> MSYSAYFAKAGFQFPAGLSALVAGIVALNVCTGRPTKGTKEISNAEYNATPIGYLQSPDQHPTAFPKVPGMKDVHGSPHHHH;> MMRAAQKAKQELPATVLTQTRSYLAPLRSDFTEEITAPKVASASNLVNEWNNKKQATENLMKLLQAYKDIGDAKSEPLLKNHNPRTFEDRDYPVPDFRTQNLKAGDVPKFFDTVISTRASAAIASKDKFWAGRKTEAEAASAKASAAFPRVAVPEWKKGKTVSIENLNTVTDKYAAALVPKRKLALPVLPEGVKKAVEDFAASVGQAKNASEVSELLAKSLAEKAVVTEGGKVVEGFSYVSKAVAAKVIATRRAEVHERLLKLWAKRLLVSPELAIVPLNEFDAQLASKFEGISPKYQELLSAVAQGNKTFAQRLNSSPAFSSFLLKREKAESEVPPSELELEAAQKAAELEDPEVALRTLLGPQMEALGASDLLLSEQIRVITEHRYTPDRLQYKEGMKLADKIAAQEAALKEELKVIYGDNVDVKHFQASPRTPVQQLFDSLKNAAANKERAAKEAAAAASPYLAYAVTKKQEVQADPSNIPFDEVLYPQLSEELLELELSDIREDEIALEKAEEEELWLLTLTQQFKHIQKHFGIDLPHSVVAHMDPLLIKKIDWETTNALEDFDITLDDMGAEDAKEQWGAENLSHHFLPLIRYRRDLARKNGDRYGPDLVNGN;> ENDVPAILKEIDSLVSREAVSAKEVSDAAVALTYLQVKANRRLWGKVLEKAGAAQDYDAASLTNLLWAINTGGVEHFKTVAELAGPAVSLLPSLSPVQLSIVVEALGGAGVKNYELYNKASAVVVSKIGEFKPAEIARVLYGVAFGGVNDVALAKAAGKVFASTEVDSRTAAQALYALAKLGRADKATVDALLKSFKKGTESASDAAAASFALGSLSFKAEKAIVDALKASAGDLAPAQAVEAAYGLALSGATDAEAFKALFGVVAPAIEKAPDALEVSSLAQLHVASTISGAKLPAAVGSFVAKAFGLAADAARLKRSSAESALVADVAAATAVAFGAQYRPEVASAVASYVKTAPDGSVLDIAITKGDAKVLVQAVPSSLLTSTTPAKPLGHVAAYSKVREAQGYAVAVVPANEFEALPDQKAKAQYVLAAIKKVAPSF;> MRQASRLALSIRQAGNVEAASAVPAMTRQFSAPGSHEHHETPLSKVMPTVVSIPRKVACLALGATKKVVCGLASSGPSQNLVSTFANKVIVEENLVNVAEIDVPFWSYWLSSAGFTSKDAFVKFAEAVKPKVAALSTSDITNLTVAFKRANYYDKDLFTGIEANVSANFTKFETEQLLQIVATFDAFNHSSVAFLDDVADSITYCNHYLAPVRAGADELATLLTYYAKNGHERADLLATVARGFSEVSLGKLSAAQRKDTVLSALKAFQTFGFYPESIEAVIGAALVSPAEYSAEELKEVEAVKVAAENALGGEFVLIQEGAHGH;> ATEPAVSKKEVLYFLSSKDAESSTAVKSYLKSLYAGAQVEATETDASELIAQLEKKYLSAQVVEPGVHNIALPLGESGSAPVKRYAAELFNLGAQAGFECPFIEVSKKFGQETATSETVKDVLNKTKSYVSADYNAALNEVLSSVEAEINGPVLFDGKTEGFKKFAAKAKAVAVSRGLPADTILAYCAGSANEDAADKVSKEFFTWFESAYTADAAAEVKAIEAEAASILDRHLAKPVAQIRKEQASAYASLLKRAETAKGAKWAEKYLEDVKAVQWFDASVAEAPASGPKVAA;> MKLLPESLQQEAATAAVVASWVLWHLDTQLLPTIMREHKLHACWAAAAKRYNEKLFKLNPSYDRVLSLPAVSKNQVLENVFHTAPKAPVEHLEKMVSANSKVYDALNLQSKRVLIWQVKPALF;> MMLRTLTRSSAVAGQAVRLFKTSAAAAEGNSVAGIIKSVNETSGANLLSSLKTIKAQAAPIYPAAASSTGYSTQAKIALFGALSWILYRADGQSKAHEWIVDLNLNVLQAAWLISFSSLIPFRAVYFAFRGMAPAT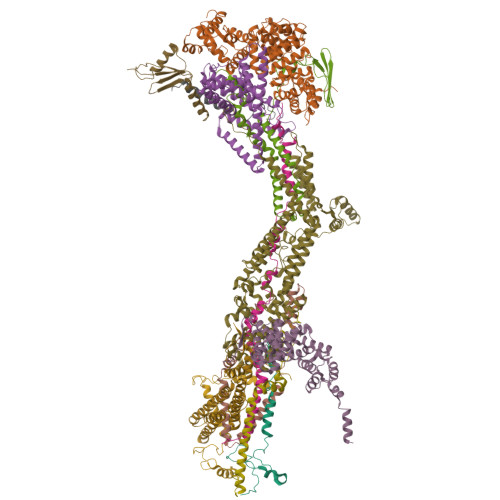ASTLNGLKTFSSISL;> MSSVRAGVEAGRRDLTTFTFSGLQDAPVAALSGSIKLNVAAKAGKAEVTVAAGAAKAATQVSAAALRKLSGSKISLAEVARISVLHSSIQNYLLSLSNERYQLLSQWPDFTTMYGKDFYYRAHPEDLKKFYDAADEYYKLYETVTEFDSLSALASQVVPNYAARRRSTVHPAIGSTVADGAFTNFLLSKQ;> MVLGEVYLKDILRTPPTGAIPANVPHPFQTSFYTYATKKLIPRHWYLLGGFTFTITLYGILDGLRDSGKKKAYDEAIHAGKTPYTAGGH;> MAVTSFLGKAFEKYFYDFSAYEQFGLNRFLSSKGQYVALRHVGFVMVGVNVLLAANFPFNPPFPTIGMCPAGWEGTWVCQADKAKALEMYKEWKKSN;> MSVLSSVSMGSRIGSSLLGRSSAYLAQCGFSTRSNLNGSIDTSSSVFQALSSDNENKPAASPLNVKLPGMSCSSILLPKTSRIAVPFGNQTMAMSSVRDVKTGSLPTNFLTGVYRFWRSQNPAEKPHDPVNDRLLPAVVDASDKRASIGTWATTFFCTIISCNLLGLMPFNEAPTSGLGFATGLGVSVWATATILGLSKTGFKFPGHFIPGGTPWPMAFIFVPLETISYTFRAVSLGVRLWVNMLAGHTLLHILTGMALALPFSLGFFSMVPATFGVCCLLSALVGLEYLVAVLQSGVFSILSTVYVGEFNHDKFIGPAAKIVKKIH;> MLARVASVALRRAEGKIMPQMVRALSVSAASAAQAELKLPTAPLQLSGTSAQIATLLWQVAAKENQLDKVQDELYQFIELFKQHSELRRLATDPFVPTLVRTKIISSVLKDSGASEITKKLFEALADEGALSALLEVTVNYEELMLAHKKEVYCTVITAEPLDKLERVELTKKAEKFVDAGFKLVMQEKIDKKLLGGFVIEFSDRRVDMSTAKKVEEFNNFVNKLVLSI;> MRSPAAFVARSGLFKASLGQSNWAQKAEQMMASVTRTFAADAKALDELRKPKFSSKYLIQHVSQKLIPAVKEWEKSYQPPVIHLGRVLSVGDGIARVYGLKSVQAGELVCFDSGVKGMALNLQADHVGVVVFGNDSVIHQGDLVYRTGQIVNVPIGPGTLGRVTDGLGQPIDGKGPLTNVRSSLVEVKAPGIIARQSVREPLFTGVKAVDALVPIGRGQRELIIGDRQTGKTAVAIDAIIHQKNCNEQVPKAQRVYCVYVAVGQKRSTVAQLVKLFTQTGAMRYTIMVSATASDAAPLQFLAPYSGCAMAEYFRDTGKHGLIIYDDLSKQSVAYRQMSLLLRRPPGREAFPGDVFYLHSRLLERAAKLSKELGGGSLTAFPVIETQAGDVSAYIATNVISITDGQIFLETELFYKGIRPALNVGLSVSRVGSAAQFPGMKQVAGTLKLELAQYREVAAFAQFGSDLDAATQYVLERGARLTEMLKQKQFAPIPIERQTVAVYAATKGFLDKVRVQDIVAAEEAVISQVNPAVFKILKANGKITPALDAHLKAELRKVKLPGA Sdk1 and Sdk2 are single-pass transmembrane proteins, with extracellular regions composed of 6 N-terminal immunoglobulin (Ig) domains followed by 13 fibronectin type III (FNIII) domains, and a relatively short intracellular domain terminating in a Postsynaptic density/Discs Large/ZO-1 (PDZ) binding motif. Here, we report the crystal structures of cell-cell adhesive homophilic dimers of mouse Sdk1 and Sdk2, each mediated by the four N-terminal Ig domains. These four domains adopt a horseshoe conformation, like many other IgSF cell-cell recognition proteins, but they interact in a unique back-to-back anti-parallel manner not previously observed. Overall, our data suggest a model in which Sdks form cis dimers on isolated cell surfaces, which dissociate to form trans dimers through the same interface when contact is made to a cell surface expressing the cognate Sdk.

Two crystal forms of Sdk1Ig1–4 were determined at 2.2 and 3.2 Å resolution respectively, one of Sdk1Ig1–5 at 3.5 Å, two of Sdk2Ig1–4 at 2.7 and 3.2 Å respectively, and one of the Sdk2Ig1–2/Sdk1Ig3–4 chimera at 2.7 Å resolution. The left hand panel shows a structural alignment of single protomers from the two different Sdk1Ig1–4 crystal forms and the Sdk1Ig1–5 structure, showing the very high structural similarity of individual protomers among the different crystal forms. The dimer protomers are related by crystallographic 2-fold symmetry in both of the Sdk1Ig1–4 structures, and by non-crystallographic symmetry in all the other structures. Although the Ig1–2:Ig1–2 interaction is present in all of the crystal forms of Sdk1 and Sdk2, there is a difference in rotational angle between the two horseshoes of the dimer among the crystal forms, with the Ig1–2:Ig1–2 interface acting as the hinge. This results in differing levels of interaction between the Ig3–4 regions in the Sdk1 and Sdk2 dimers in the different crystal forms. The Ig3–4:Ig3–4 interaction varies from the Ig3–4 domains forming a considerable additional interface—as in Sdk1Ig1–4 crystal form 2 (915 Å2 BSA) and Sdk2Ig1–4 crystal form 1 (1294 Å2 BSA)—to being splayed 14 Å apart, as in the Sdk1Ig1–4 crystal form 1 structure (0 Å2 BSA). These differences indicate that there is flexibility in the interaction between the horseshoes in solution, with different conformations being trapped in the crystals.

> GPALAQDDVAPYFKTEPGLPQIHLEGNRLVLTCLAEGSWPLEFKWIRNDSELTTYSSEYKYIIPSLQKLDAGFYRCVVRNRMGALLQRKSEIQVAYMGNFMDTDQRKTVSQGHAALLNLLPIVSCPQPQVTWFREGHKIIPSSRIAITLENQLVILATTASDAGAYYVQAVNEKNGENKTSPFIHLSVARDTGTHEAMAPIIVVAPGNRSVVAGSSETTLECIANARPVEELSVHWKRNGVRLTSGLHSYGRRLTITNPTSADTGMYVCEATLRGSTFEPARARAFLSIIEPPYFTAEPESRILGEVEETMDIPCRAMGVPLPTLQWYKDAVPLSKLQNPRYKVLPSGGLHIQKLSPEDSGIFQCFASNEGGEVQTHTYLDVTN>[4x]CYCRIPA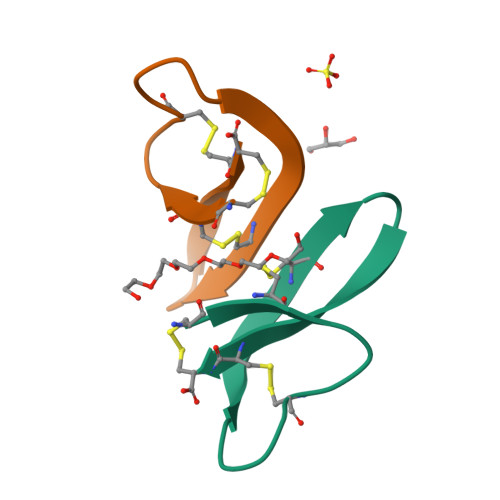CIAGERRYATCIYQGRLWAFCC> MAVPFVEDWDLVQTLGEGAYGEVQLAVNRVT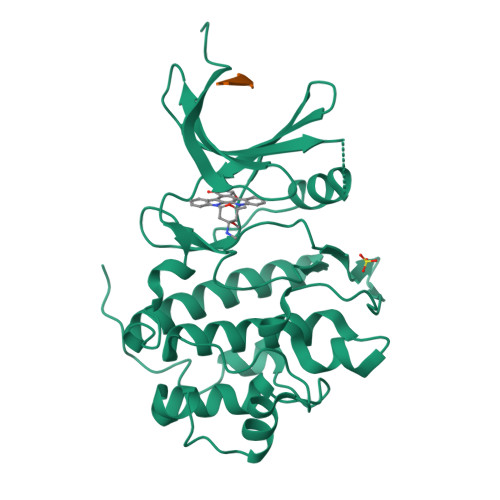EEAVAVKIVDMKRAVDCPENIKKEICINKMLNHENVVKFYGHRREGNIQYLFLEYCSGGELFDRIEPDIGMPEPDAQRFFHQLMAGVVYLHGIGITHRDIKPENLLLDERDNLKISDFGLATVFRYNNRERLLNKMCGTLPYVAPELLKRREFHAEPVDVWSCGIVLTAMLAGELPWDQPSDSCQEYSDWKEKKTYLNPWKKIDSAPLALLHKILVENPSARITIPDIKKDRWYNKPLKKGAKRPRVTSGGVSESPSG;> ASVSA(5S)-5-(3-{4-[(2-chloro-4-fluorophenoxy)methyl]piperidin-1-yl}-3-oxopropyl)pyrrolidin-2-one | 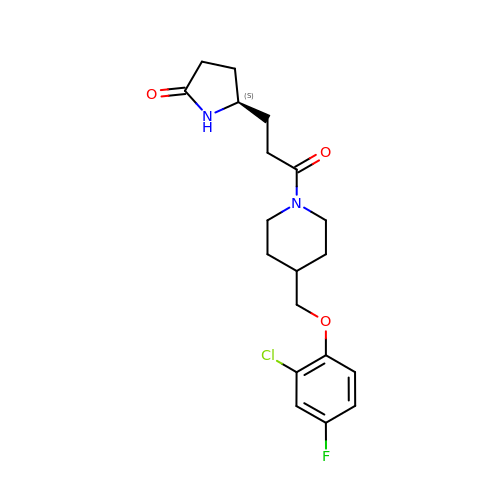C19 H24 Cl F N2 O3 | AKWBGFHQJGRBNZ-HNNXBMFYSA-N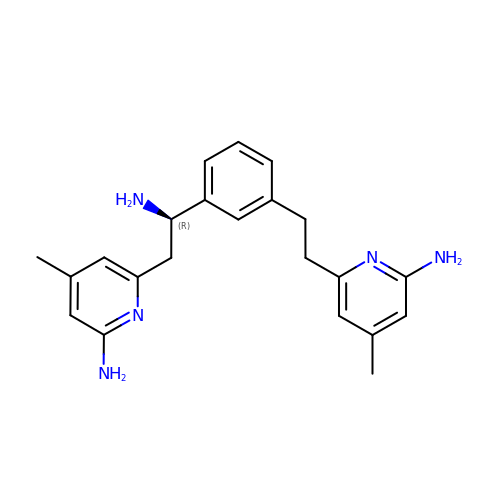(R)-6-(2-Amino-2-(3-(2-(6-amino-4-methylpyridin-2-yl)ethyl)phenyl)ethyl)-4-methylpyridin-2-amine | C22 H27 N5 | HPGDXHOKQNTRIC-HXUWFJFHSA-N> MNHPLFTEGTYQAEV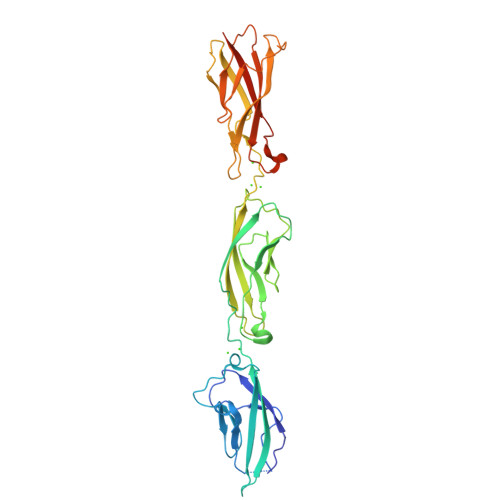MENSPAGTPLTVLNGPILALDADEDVYAVVTYQLLGTHSDLFVIDNSTGVVTVRSGIIIDREAFSPPFLELLLLAEDIGQLNGTAHLFITILDDNDNWPTFSPPTYTVHLLENCPPGFPVLQVTATDEDSGLNGELVYRIEAGAQDRFLIHPVTGVIRVGNATIDREEQESYRLTVVATNRGTVPLSGTAIVTILIDDINDSRPEFLNPIQTVSVLESAEPGTIIANVTAIDLDLNPKLEYHIISIVAKDDTDRLVPDQEDAFAVNINTGSVMVKSPLNRELVATYEVTLSVIDNASDLPEHSVSVPNAKLTVNILDVNDNLEHHHHHH>[3x]TPASGALLQQMNLASQSLNYELSFISINKQGVESLRYRHARLDNRPLAQLLQMDGPRREVVQRGNEISYFEPGLEPFTLNGDYIVDSLPSLIYTDFKRLSPYYDFISVGRTRIADRLCEVIRVVARDGTRYSYIVWMDTESKLPMRVDLLDRDGETLEQFRVIAFNVNQDISSSMQTLAKANLPPLLSVPVGEKAKFSWTPTWLPQGFSEVSSSRRPLPTMDNMPIESRLYSDGLFSFSVNVNRA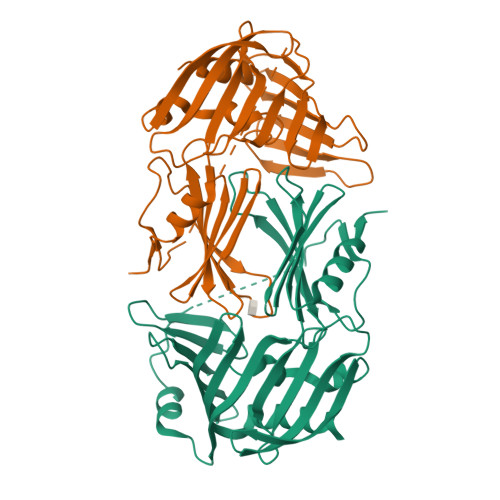TPSSTDQMLRTGRRTVSTSVRDNAEITIVGELPPQTAKRIAENIKFGAAQ GUANOSINE-5'-RP-ALPHA-THIO-TRIPHOSPHATE | C10 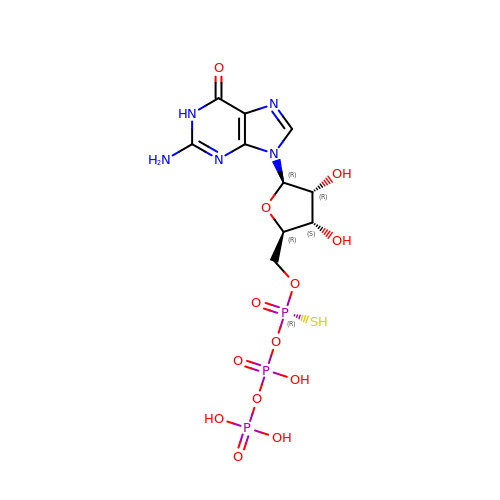H16 N5 O13 P3 S | YRUWXBKVSXSSGS-KIOICMOXSA-N>MADTKAKLTLNGDTAVELDVLKGTLGQDVIDIRTLGSKGVFTFDPGFTSTASCESKITFIDGDEGILLHRGFPIDQLATDSNYLEVCYILLNGEKPTQEQYDEFKTTVTLHTMIHEQITRLFHAFRRDSHPMAVMCGITGALAAFYHDSLDVNNPRHREIAAFRLLSKMPTMAAMCYKYSIGQPFVYPRNDLSYAGNFLNMMFSTPCEPYEVNPILERAMDRILILHADHEQNASTSTVRTAGSSGANPFACIAAGIASLWGPAHGGANEAALKMLEEISSVKHIPEFFRRAKDKNDSFRLMGFGHRVYKNY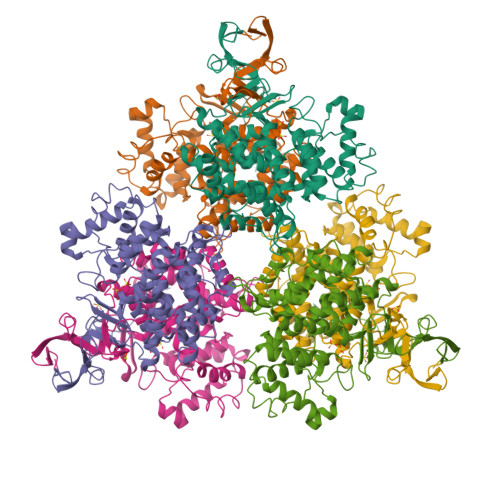DPRATVMRETCHEVLKELGTKDDLLEVAMELENIALNDPYFIEKKLYPNVDFYSGIILKAMGIPSSMFTVIFAMARTVGWIAHWSEMHSDGMKIARPRQLYTGYEKRDFKSDIKR[2x]> ASQKVEKTVIKNETGTISISQLNKNVWVHTELGSFNGEAVPSNGLVLNTSKGLVLVDSSWDDKLTKELIEMVEKKFQKRVTDVIITHAHASRIGGI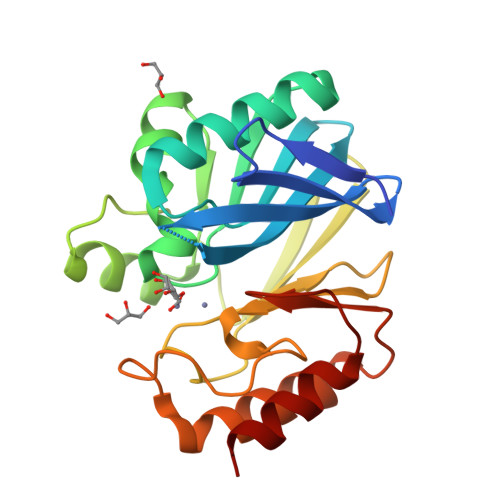KTLKERGIKAHSTALTAELAKKNGYEEPLGDLQTVTNLKFGNMKVETFYPGKGHTEDNIVVWLPQYNILVGGCLVKSTSAKDLGNVADAYVNEWSTSIENVLKRYRNINAVVPGHGEVGDKGLLLHTLDLLK4-[[(2~{S})-oxolan-2-yl]methyl]-3-pyridin-3-yl-1~{H}-1,2,4-triazole-5-thione | C12 H14 N4 O S | 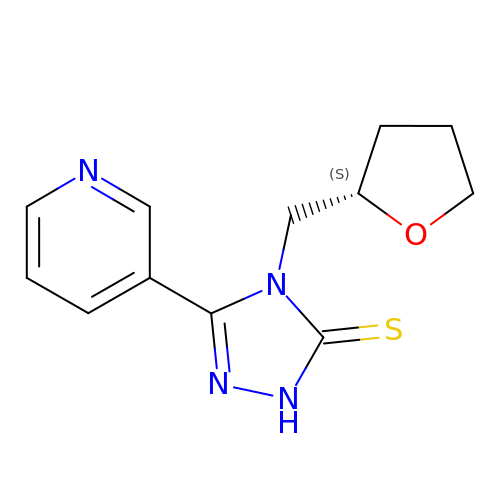UPESTZWCQNGAJI-JTQLQIEISA-N2-{[(2S)-1-amino-5-{[(1Z)-2-chloroethanimidoyl]amino}-1-oxopentan-2-yl]carbamoyl}benzoic acid | C15 H19 Cl N4 O4 | 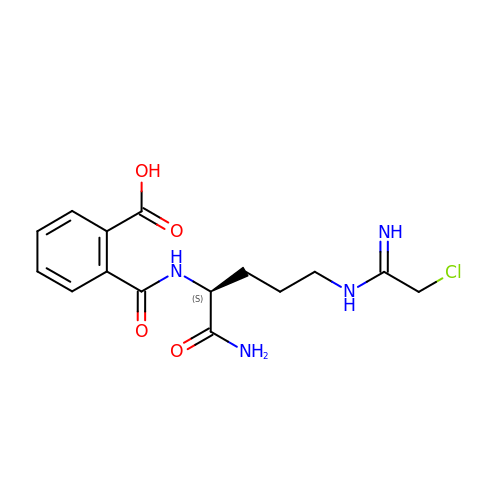VUCFCRGOVAAFJN-NSHDSACASA-N>[2x]MAAPDLLDPKSATHNTKPRLSFSSKPIVYNSGDDCESITTVMKWKTVLAIFLLVVLYLIIGATVFKALEQPEEGLQKYRIIQEKIDFLSMHTCVQTSELEDLVKQVVLAIRAGVNPSGH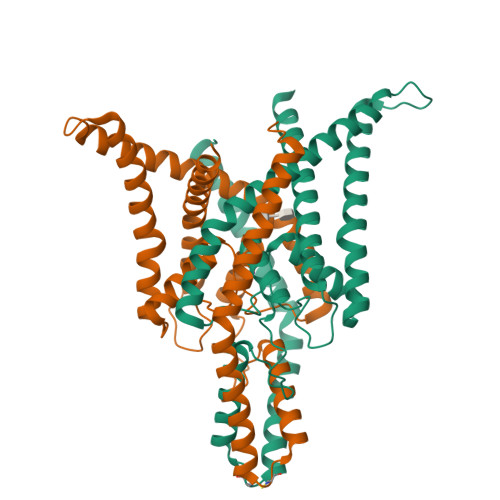PSQESSMWDLSSSFFFAGTVITTIGFGNVSPHTEGGRIFCIIYALLGIPLFGFLLAGVGDQLGTIFGKGIAKVEKMFVKWNVSQTKIRVTSTVLFILFGCLLFVALPALIFQHIEGWSALESIYFVVITLTTIGFGDFVAGGSEIEYLDYYKPIVWFWILVGLAYFAAVLSMIGDWLRVISKKTKEEVGEFRAHAAEWTANV N-[5-[2-[(1S)-1-cyclopropylethyl]-7-[[4-[(dimethylamino)methyl]phenyl]sulfamoyl]-1-oxidanylidene-3H-isoindol-5-yl]-4-methyl-1,3-thiazol-2-yl]ethanamide 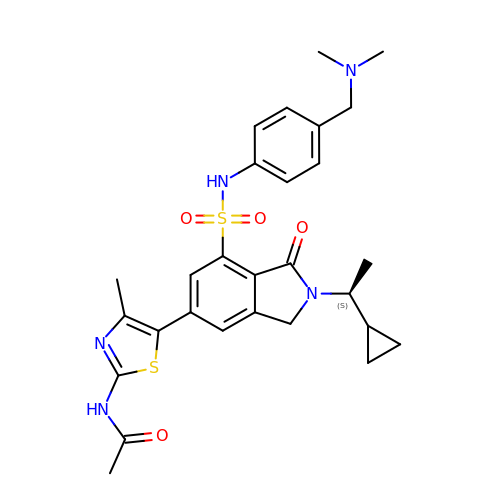| C28 H33 N5 O4 S2 | OMXQWLDNOXGCSM-KRWDZBQOSA-N> MKISIGLGKEGVEERLAERGVSRRDFLKFCTAIAVTMGMGPAFAPEVARALMGPRRPSVVYLHNAECTGCSESVLR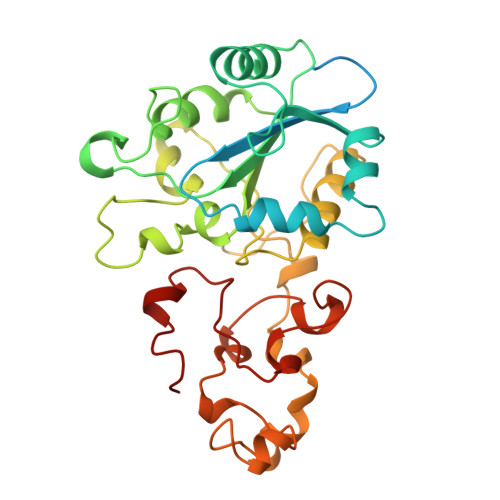AFEPYIDTLILDTLSLDYHETIMAAAGDAAEAALEQAVNSPHGFIAVVEGGIPTAANGIYGKVANHTMLDICSRILPKAQAVIAYGTCATFGGVQAAKPNPTGAKGVNDALKHLGVKAINIAGCPPNPYNLVGTIVYYLKNKAAPELDSLNRPTMFFGQTVHEQCPRLPHFDAGEFAPSFESEEARKGWCLYELGCKGPVTMNNCPKIKFNQTNWPVDAGHPCIGCSEPDFWDAMTPFYQN> SEDAGLVAEAEAVAAGWMLDFLCLSLCRAFRDGRSEDFRRTRNSAEAIIHGLSSLTACQLRTIYICQFLTRIAAGKTLDAQFENDERITPLESALMIWGSIEKEHDKLHEEIQNLIKIQAIAVCMENGNFKE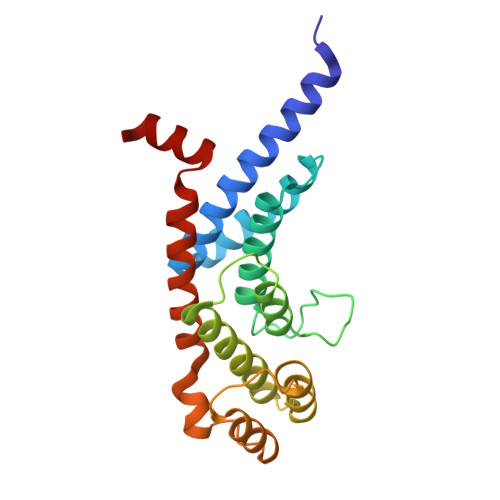AEEVFERIFGDPNSHMPFKSKLLMIISQKDTFHSFFQHFSYNHMMEKIKSYVNYVLSEKSSTFLMKAAAKVVE>PMFIVNTNVPRASVPDGFLSELTQQLAQATGKPPQYIAVHVVPDQGMAFGGSSEPCALCSLHSIGKIGGAQNRS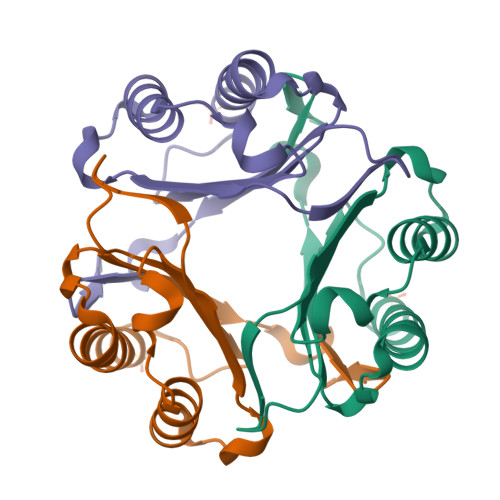YSKLLCGLLAERLRISPDRVYINYYDMNAANVGWNNSTFA[3x]>[4x]GMKRKIIYLASPYGFSQQQKTLLLPPIVRALEALGIEVWEPFARNNQIDFSQADWAYRVAQADLQDVKNCDGIFAVVNGTPPDEGVMVE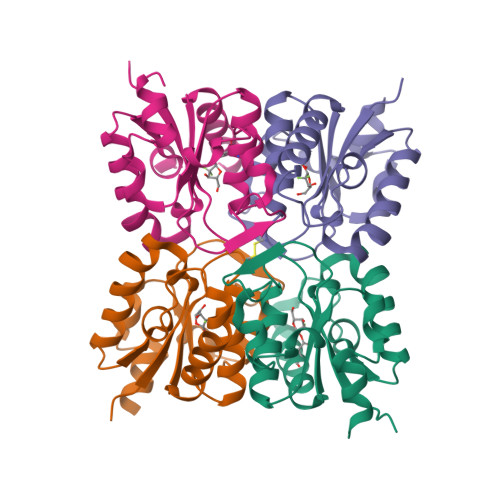LGMAIALNKAIFLFRDDFRRCSDNERYPLNLMLFAGLPEIGWENYYYTSVDEIQSHDKALYKWLTGM>[4x]GKHYKRPQDELPCNEYSQPGGDGSYVSVPSPLGKIKSMTKEKADILLLRAGLPSHFHLQLSEIEFHEIIGSGSFGKVYKGRCRNKIVAIKRYRANTYCSKSDVDMFCREVSILCQLNHPCVIQFVGACLNDPSQFAIVTQYISGGSLFSLLHEQKRILDLQSKLIIAVDVAKGMEYLHNLTQPIIHRD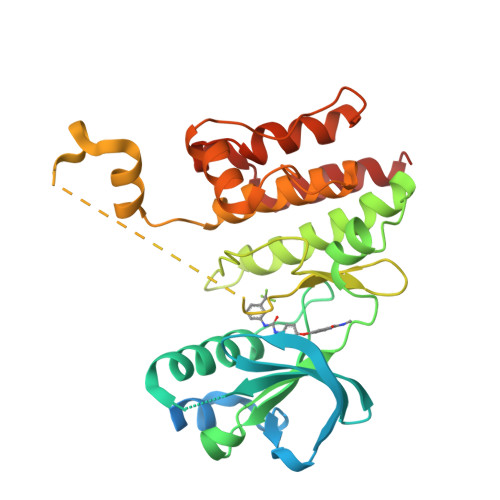LNSHNILLYEDGHAVVADFGESRFLQSLDEDNMTKQPGNLRWMAPEVFTQCTRYTIKADVFSYALCLWEILTGEIPFAHLKPAAAAADMAYHHIRPPIGYSIPKPISSLLIRGWNACPEGRPEFSEVVMKLEECLCNIELMS A major challenge in the further development of nucleoside analogues for therapeutic applications is access to scalable and environmentally sustainable synthetic strategies. This study uses the type II nucleoside 2′-deoxyribosyltransferase from Lactobacillus leichmannii (LlNDT-2) to prepare a suite of ribonucleoside analogues using naturally-occurring uridine and cytidine sugar donors. An enzymatic alternative to the use of NPs to prepare ribonucleoside analogues is to use nucleoside 2′-deoxyribosyltransferases (NDTs). These enzymes catalyse the formation of nucleoside analogues via an overall nucleobase exchange much akin to NPs. However, NDTs are mechanistically distinct, forming a covalent adduct within the active site, thus controlling stereoselective nucleophilic attack of the incoming nucleobase on the β face.

To gain further insight into how the presence of a 2′-OH substituent on the ribonucleoside donor influences substrate recognition and subsequent catalytic steps, structural studies were conducted on the wildtype LlNDT-2 and a double mutant Y7F/D72N. To explore the structural implications of the differences between the two enzymes, WT-LlNDT-2 and the Y7F/D72N mutant were both crystallised using conditions determined for the WT-LlNDT-2 enzyme previously. Complexes were obtained by soaking cytidine 8 into the crystals. All structures contained two molecules in the asymmetric unit, constituting one third of the hexamer routinely observed in solution. In the case of WT-LlNDT-2, electron density in the omit maps obtained could be clearly modelled as the ribosylated intermediate, and the cleaved cytosine nucleobase, whereas in the Y7F/D72N structure cytidine 8 was intact, presumably reflective of its poorer kcat as observed for CtNDT. By contrast, the ribosylated intermediate of CtNDT reported by Tang and co-workers32 features the ribose flipped approximately 90° from this position, with the 2′-OH interacting with the side chain of D62 (D72 in LlNDT-2), despite the conservation of most active site residues, although the authors report multiple conformations of the ligand in this complex, evidenced by ambiguous electron density. Therefore, despite previous studies highlighting that WT-LlNDT-2 ribonucleosides are poor substrates, this can be overcome by increasing the enzyme loading.

>MPKKTIYFGAGWFTDRQNKAYKEAMEALKENPTIDLENSYVPLDNQYKGIRVDEHPEYLHDKVWATATYNNDLNGIKTNDIMLGVYIPDEEDVGLGMELGYALSQGKYVLLVIPDEDYGKPINLMSWGVSDNVIKMSQLKDFNFNKPRFDFYEGAVY[2x]The type VI secretion system (T6SS) is a recently discovered protein transport complex which contributes to bacterial pathogenesis. Secreted proteins of E. tarda T6SS include a Hcp homolog EvpC, a VgrG homolog EvpI, and a novel protein EvpP which is not commonly present in other T6SS clusters. Our previous functional studies showed that the major secreted protein EvpC is a key member in the EVP system of E. tarda and the secretion of EvpC is a critical step for the function of T6SS. The overall structural and sequence similarity between EvpC and Hcp1 strongly suggest that EvpC is a member of the Hcp family of proteins.

The structure of recombinant EvpC from E. tarda was solved by molecular replacement using a dataset collected on an R-axis rotating anode generator and refined to a 2.8 Å resolution. The EvpC model consists of residues from Ala2 to Lys163. There are two molecules in the asymmetric unit. These two molecules are part of two hexameric rings which can be generated using crystallographic symmetry. Each monomer of EvpC consists mainly of a β-barrel domain, with extended loops lying predominantly on one side of the β-barrel. The diameter of the monomeric β-barrel is approximately 12 Å consisting of 11 anti-parallel β-strands. In addition, an α-helix (Ala66 - Gln76) is located on one side of the β-barrel. Residues Gly35 to Met53 form an extended loop which protrudes approximately 20 Å from the β-barrel. A head-to-head stacked hexameric ring structure of EvpC can be observed in the crystal lattice. This stacked ring structure forms a tube with an outer diameter of 80 Å and an inner diameter of 40 Å. The analysis of crystal structure confirms that all these residues (D4, E15, E26, K161, K162 and K163) are exposed on the outer rim of the EvpC hexameric ring which makes them available for interaction with other proteins.

>[2x]MAFDTYIKLDKVDGESTDDKHKKWIEVLGFAWGAGNECTMESGTQGLNTGKAMMSVLRVTKWMDCASVKLASAAVQGQNFPTLELEICTQAGDKFAFCIYKFTHVAVSSYQCSGATGGSDRPQETIDFAYKEVTWEYVPQDQNGKAGGKIGPEGWSLITNKKK> MHHHHHHHTGAAPDRKAPVRPTPLDRVIPAPASVDPGGAPYRITRGTHIRVDDSREARRVGDYLADLLRPATGYRLPVTAHGHGGIRLRLAGGPYGDEGYRLDSGPAGVTITARKAAGLFHGVQTLRQLLPPAVEKDSAQPGPWLVAGGTIEDTPRYAWRSAMLDVSRHFFGVDEVKRYIDRVARYKYNKLHLHLSDDQGWRIAIDSWPRLATYGGSTEVGGGPGGYYTKAEYKEIVRYAASRHLEVVPEIDMPGHTNAALASYAELNCDGVAPPLYTGTKVGFSSLCVDKDVTYDFVDDVIGELAALTPGRYLHIGGAEAHSTPKADFVAFMKRVQPIVAKYGKTVVGWHQLAGAEPVEGALVQYWGLDRTGDAEKAEVAEAARNGTGLILSPADRTYLDMKYTKDTPLGLSWAGYVEVQRSY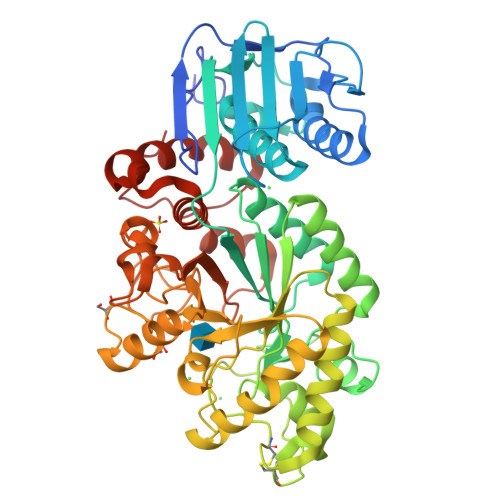DWDPAGYLPGAPADAVRGVEAPLWTETLSDPDQLDYMAFPRLPGVAELGWSPASTHDWDTYKVRLAAQAPYWEAAGIDFYRSPQVPWT> MGSSHHHHHHSSGENLYFQGHMVDLRSDTVTRPGPAMRRAMAEAVVGDDDYGEDPTVHELQEKAAELLGVERTLFVPTNTMANLISVMGHCRRRGSQVLLGQECHLHVYEQGGVAQIAGVHSHPLPDLPYGTLDLNELERALTRGSGSPYHPVCELVYLENTHSSAGGRVLPVDYLRQVCLLAHAHGARVHMDGARLMNAAVALRIPPARLVEHCDSVSFCFSKGLGAPVGALVGGSKDFIGEAWRLRKALGGGMRQAGVLAAAALVGLAEAEEVLPRDHENAQRFAKGLQDLASPICSVDPATVETNMVLVQVAGLPPSELCQRLQAVSAEEVAQTGRAVRVLLFPWTEQSVRAVWHRDVSAQDTELALKKWEFVLRQLRP

Reactions 1 and 4 are catalyzed by two Fe2+-dependent dioxygenases: TML dioxygenase (TMLD) and γ-butyrobetaine dioxygenase (BBD), which are related by homology; reaction 3 is catalyzed by trimethylamino butyraldehyde dehydrogenase (TMABADH); reaction 2, the aldol cleavage of HTML to generate glycine and TMABA, is catalyzed by HTMLA. However, a mouse protein absent in humans (threonine aldolase; Tha1) catalyzes the reaction more efficiently. However, the preferred substrate of Tha1 is HTML with a catalytic efficiency in the order of 104 s−1 M−1, followed by L-allo-threonine (102 s−1 M−1) and L-threonine (101 s−1 M−1). As we found that the mouse enzyme has a strong preference (1000 folds) for HTML towards threonine, the name hydroxytrimethyllysine aldolase (Htmla) would be a better descriptor of the mouse gene.

To verify if the results of our screening for Tha1 are confirmed or improved with the availability of an experimental structure, we decided to determine the crystal structure of mouse Tha1. Mouse Tha1 crystallizes in two space groups, in orthorhombic F222 and in monoclinic C2, with one molecule and two molecules in the ASU, respectively. Tha1 did not rank highest based on the AlphaFold model, but its rank improved to second place using the experimental crystal structure we determined at 2.26 Å resolution. The PLP cofactor is visible only in the monoclinic structure; however, the active site is very similar in the two cases, with only minor differences. The expected tetrameric quaternary structure is formed by crystallographic symmetries, with four identical units in F222 (related by a 222 symmetry) and two identical dimers in C2 (related by a two-fold axis). The RMSD values between the single units (around 0.26–0.28 Å) indicate that the monoclinic and orthorhombic structures are similar. Also the tetrameric assembly is conserved in the two space groups, with two main interfaces. As indicate by data from PISA analysis, the interface between units A and B (analogous to that between units C and D, termed “main interface”) is contributing stronger to the stability of the quaternary structure in comparison with the interface between units A and C (analogous to that between units B and D, termed “secondary interface”). Hence, the tetramer can be considered a dimer (AB + CD) of dimers (A + B and C + D), with the first dissociation being ABCD to AB + CD (as determined by PISA). Interestingly, the Tha1 ranking in our screening greatly improved by using the crystal structure of the mouse protein or AlphaFold models built taking this information into account.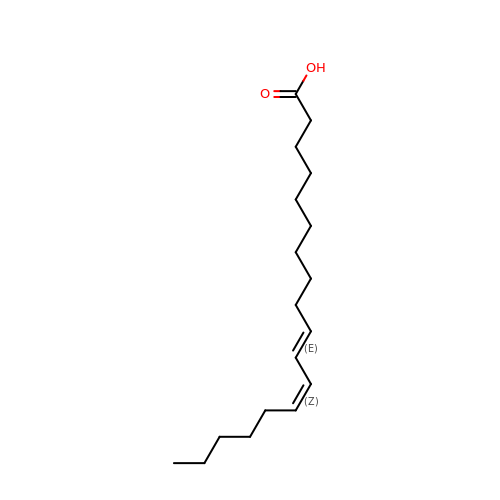(10E,12Z)-OCTADECA-10,12-DIENOIC ACID | C18 H32 O2 | GKJZMAHZJGSBKD-NMMTYZSQSA-N>MTMEKGMSSGEGLPSRSSQVSAGKITAKELETKQSYKEKRGGFVLVHAGAGYHSESKAKEYKHVCKRACQKAIEKLQAGALATDAVTAALVELEDSPFTNAGMGSNLNLLGEIECDASIMDGKSLNFGAVGALSGIKNPVSVANRLLCEGQKGKLSAGRIPPCFLVGEGAYRWAVDHGIPSCPPNIMTTRFSLAAFKRNKRKLELAERVDTDFMQLKKRRQSSEKENDSGTLDAVGAVVVDHEGNVAAAVSSGGLALKHPGRVGQAALYGCGCWAENTGAHNPYSTAVSTSGCGEHLVRTILARECSHALQAEDAHQALLETMQNKFISSPFLASEDGVLGGVIVLRSCRCSAEPDSS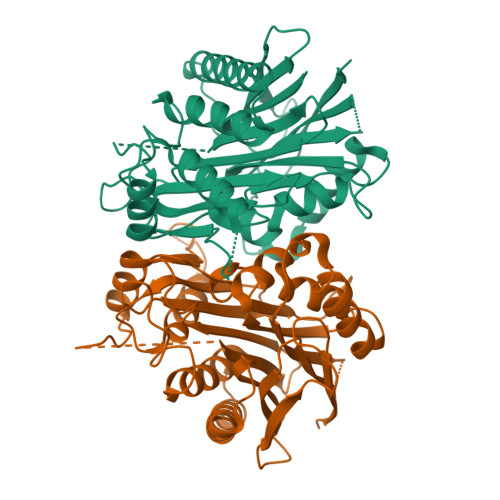QNKQTLLVEFLWSHTTESMCVGYMSAQDGKAKTHISRLPPGAVAGQSVAIEGGVCRLESPVN[2x]>SADVAGAVIDGASLSFDILKTVLEALGNVKRKIAVGVDNESGKTWTALNTYFRSGTSDIVLPHKVPHGKALLYNGQKDRGPVATGAVGVLAYLMSDGNTLAVLFSVPYDYNWYSNWWNVRIYKGKRRADQRMYEELYYNL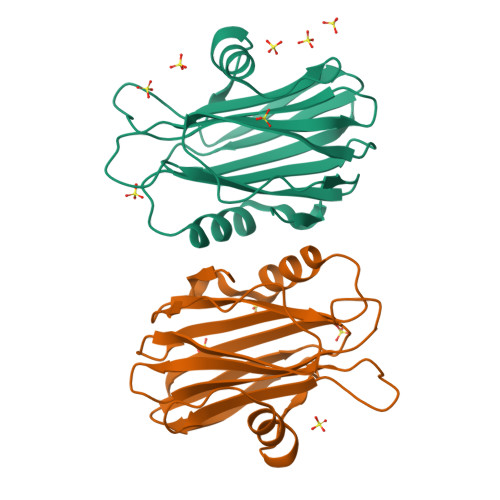SPFRGDNGWHTRNLGYGLKSRGFMNSSGHAILEIHVSKA[2x]>MHHHHHHENLYFQGSPNYDKWEMERTDITMKHKLGGGQYGEVYEGVWKKYSLTVAVK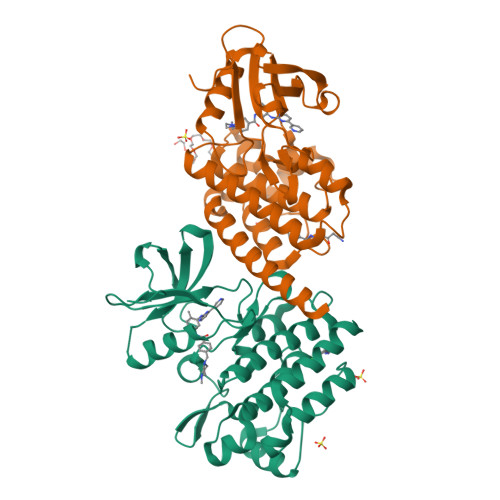TLKEDTMEVEEFLKEAAVMKEIKHPNLVQLLGVCTREPPFYIITEFMTYGNLLDYLRECNRQEVNAVVLLYMATQISSAMEYLEKKNFIHRDLAARNCLVGENHLVKVADFGLSRLMTGDTYTAHAGAKFPIKWTAPESLAYNKFSIKSDVWAFGVLLWEIATYGMSPYPGIDLSQVYELLEKDYRMERPEGCPEKVYELMRACWQWNPSDRPSFAEIHQAFETMFQESSISDEVEKELGK[2x]>MITYNDFSKIDIRVGIIKEVSDFKEAIKPAYKLKIYFGDIIGYKNSSAQITNYKKDELINKKIIAVV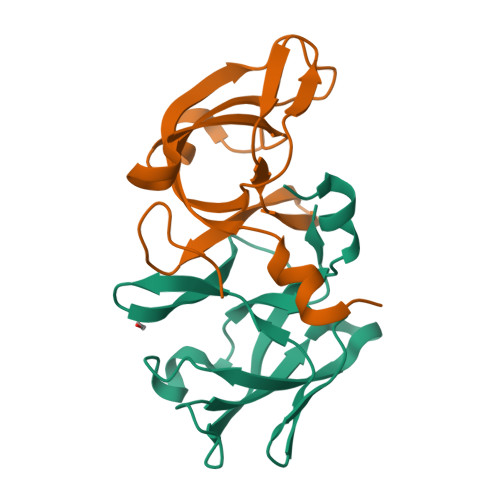NFPPKQIANFISEVLVLGAITGDGVKLLTPDGGEPGDKIA[2x]>QTPLLQNVYNRESTLLNGNWKYVIDPYETGYRNHRNWIPFDQMESTKNSAKPYYTDKVIKERWDRVEYNFNTSAEIKVPGDWNSQDRMLLYYEGSLWYRTKFDYTITDNNRLFIYFGAAN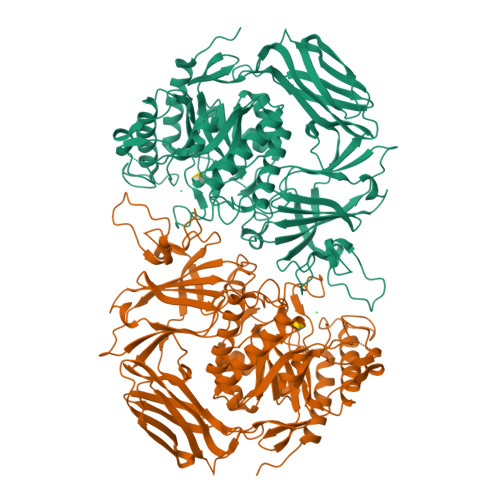YQTDVYVNGQKVGQHLGGFDPFNFDITNVVKPKDNSLMVRVDNRREKHRVPNYTTDWWNYGGITRDVKLVEVPSTYIQDYAIQLDKDNPKNIKGYVQLAGSSLETNVSINIPEAKINFSTTTDRTGRVHFEIPAKKIKKWYPKRPKLYDVQIQAGNDKLEDQIGLRTIETKGADILLNGQSIFLRGISLHEENPIKIGRARSIEDAQMQMGWAKELNCNFIRLAHYPHNENMPRLADKLGLLLWEEIPVYWGIDYENPEAFAQAKSQLETMVHRDKNRASVIVWSVANETPDTESRLEFLRQLKKIAIDIDNTRFISAALERNEKDVQDVVKIPDPFAEDVDMLACNEYIGWYSGLPEKCDKVTWQLPEDKPFFVSEFGGGALYNHHGDKLTRWTEEYQEYLYQEQIKMLKKIPTLRGMTPWILVDFRSPRRNLPIIQDGWNRKGLISDGGFKKKAFHVLKAYYDEMEKKYNYQIKDLEHHHHHH[4x]>[2x]MSPIPLPVTDTDDAWRARIAAHRADKDEFLATHDQSPIPP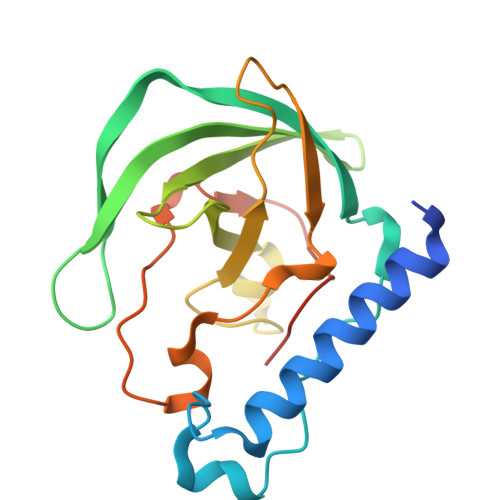ADRGAFDGLRYFDIDASFRVAARYQPARDPEAVELETTRGPPAEYTRAAVLGFDLGDSHHTLTAFRVEGESSLFVPFTDETTDDGRTYEHGRYLDVDPAGADGGDEVALDFNLAYNPFCAYGGSFSCALPPADNHVPAAITAGERVDADLEHHHHHH> MTENILRKSDEEIQKEITARVKALESMLIEQGILTTSMIDRMAEIYENEVGPHLGAKVVVKAWTDPEFKKRLLADGTEACKELGIGGLQGEDMMWVENTDEVHHVVVCTLCSCYPWPVLGLPPNWFKEPQYRSRVVREPRQLLKEEFGFEVPPSKEIKVWDSSSEMRFVVLPQRPAGTDGWSEEELATLVTRESMIGVEPAKAVAHHHHHH;> MNGVYDVGGTDGLGPINRPADEPVFRAEWEKVAFAMFPATFRAGFMGLDEFRFGIEQMNPAEYLESPYYWHWIRTYIHHGVRTGKIDLEELERRTQYYRENPDAPLPEHEQKPELIEFVNQAVYGGLPASREVDRPPK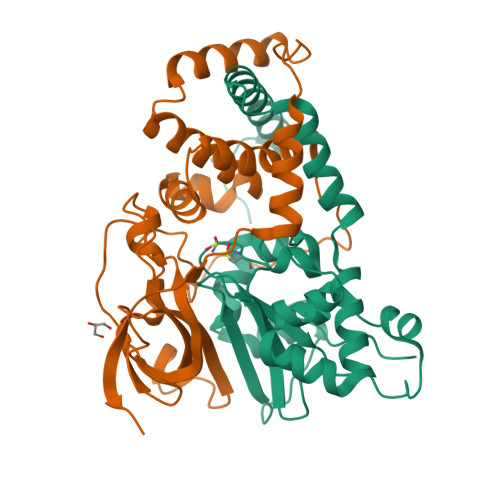FKEGDVVRFSTASPKGHARRARYVRGKTGTVVKHHGAYIYPDTAGNGLGECPEHLYTVRFTAQELWGPEGDPNSSVYYDCWEPYIELVDTKAAAA>VLDGPYQPVTFKPPNDYWILINSNSNGVVLEGTNNTDVWVAIISIEPNVNSESRQYSLFGVNKQITVVNTSNKWKFMEMFRNNSNAEFQHKRTLTSSTKLVGILKHGGRLWTYHGETPNATTDYSTTSNLNEISVTTYAEFYIIPRSQESKCTEYINTGL[2x]

Rotaviruses (RVs) are a major cause of severe gastroenteritis in children under the age of 5, causing 200,000 deaths[1–3]and account for 2 million childhood hospital admissions with an estimated cost of over 1 billion US dollars per year. It has been shown that RV attachment to cell surface carbohydrates, mediated by the VP8* domain of the spike protein VP4, is a required first step of an effective infection. Similar to other known VP8* structures, P[19]VP8*s adopted a classical galectin-like fold with two twisted antiparallel β-sheets consisting of strands A, L, C, D, G, H and M, B, I, J, K, respectively. The structural data showed that the P VP8* uses a completely new binding site that is different from the one of other RVs and this single binding site is able to interact with either type I HBGA pentasaccharide Lacto-N-fucopentaose I (LNFP I) or mucin core 2 glycan with a similar binding mode. The common shallow cleft between the two β-sheets where the glycan-binding sites of other known RVs are located is wide in P similar to the P and P /P VP8*s but wider than the P /P and P VP8*s. It was noted that the P glycan binding site is located away from the cleft and thus represents a completely new glycan binding site, consistent with our previous observations based on NMR and mutagenesis studies.

The crystal structures of P VP8* in complex with LNFP I and mucin core 2 were solved at 1.94 Å and 1.90 Å, respectively. P VP8* binds mucin core 2 using the same binding site through an almost identical conformation as that of bind LNFP I, with a RMSD 0.118 Å for the alpha carbon backbone atoms. Two amino acids, T184 and T216, which are involved in binding to LNFP I, did not participate in binding to the shorter mucin core 2 trisaccharide. The GalNAc (GalNAc-I) forms hydrogen bonds with G171 and R172, while the Gal (Gal-II) makes hydrophobic interactions with G170 and G171. The amino acid residue of threonine that links to GalNAc-I pointed into the solvent. Interestingly, the GlcNAc (GlcNAc-III) inserted into the same deep binding pocket that binds the GlcNAc-III of LNFP I. It was noted that H169 contributed to the mucin core 2 binding interaction with GlcNAc-III, but this interaction was not seen with GlcNAc of LNFP I. The GlcNAc-III was further stabilized by two amino acids (T185, R209) through hydrogen bonding interactions. Finally, it was noticed that there is a slightly shifted orientation of the GlcNAc-containing motif inside the binding pocket between mucin core 2 and the type 1 HBGAs, leading to a significant orientation shift of the backbones between mucin core 2 and type 1 HBGA within the binding cleft. This indicated a mechanism for how P VP8* is able to achieve a broader binding specificity to the extended molecules of the two glycan types.> KVQLKGRDLLTLKNFTGEEIKYMLWLSADLKFRIKQKGEYLPLLQGKSLGMIFEKRSTRTRLSTETGFALLGGHPCFLTTQDIHLGVNESLTDTARVLSSMADAVLARVYKQSDLDTLAKEASIPIINGLSDLYHPIQILADYLTLQEHYSSLKGLTLSWIG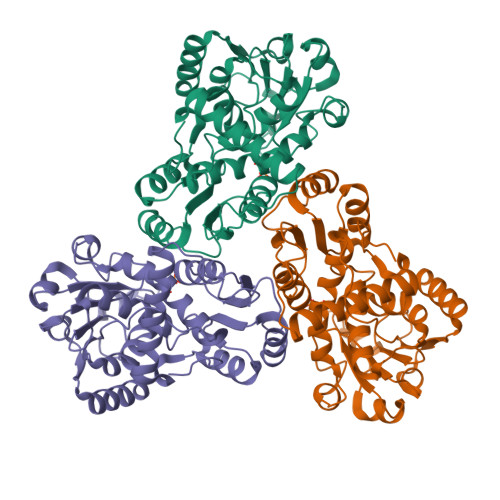DGNNILHSIMMSAAKFGMHLQAATPKGYEPDASVTKLAEQYAKENGTKLLLTNDPLEAAHGGNVLITDTWISMGREEEKKKRLQAFQGYQVTMKTAKVAASDWTFLHCLPRKPEEVDDEVFYSPRSLVFPEAENRKWTIMAVMVSLLTDYSPQLQKPKF>[2x]MGSDKIHHHHHHMFLVISVVGSSNIDIVLKVDHFTKPGETQKAIEMNVFPGGKGANQAVTVAKIGEKGCRFVTCIGNDDYSDLLIENYEKLGITG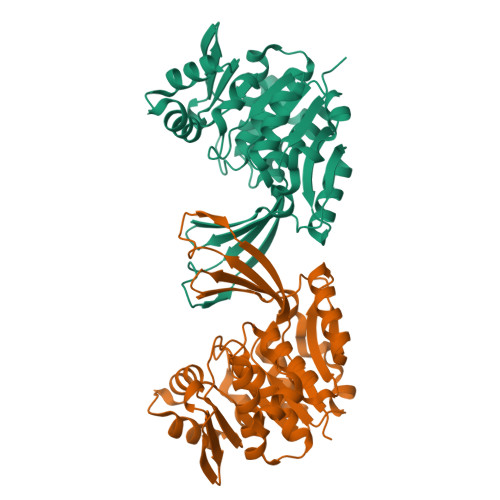YIRVSLPTGRAFIEVDKTGQNRIIIFPGANAELKKELIDWNTLSESDILLLQNEIPFETTLECAKRFNGIVIFDPAPAQGINEEIFQYLDYLTPNEKEIEALSKDFFGEFLTVEKAAEKFLELGVKNVIVKLGDKGVLLVNKNEKKHFPTFKVKAVDTTAAGDVFNGAFAVALSEGKNPEEAVIFGTAAAAISVTRLGAQSSIPAREEVEAFLKNL> MTAPILLLDGASMWFRSYFGVPSSIKAPDGRPVNAVRGFIDAISTLVTREKPRRLVVCRDDDWRPQWRVDLIPSYKAHRVAEPEPDGVPDIEEVPDDLTPQVNMILELLDAFGIPTAGAAGFEADDVLGTLSAREERDPVVVVSGDRDLLQLVRDEPAPQVRVLYLGRGLAKATKWGPAEVAEQYGVPLDRAGTAYAELALLRGDPSNGLPGVAGIGEKTAASLLAKHGSLQNILDAAHDPKSGLSKAHRTKLLGAVDYIAA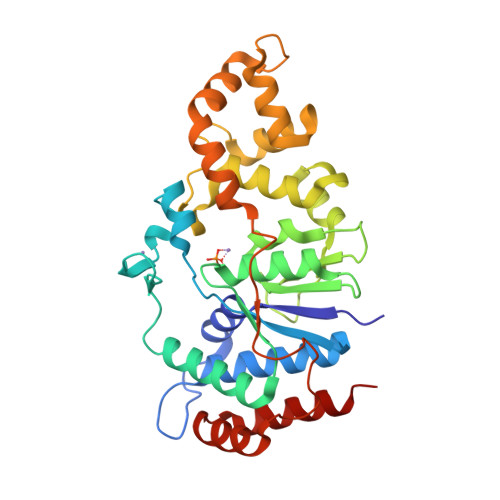AETVVRVATDAPVTFSTPTDTLPLAAGDPARVAELAAAYGVSSSISRLQTALDQLPD>MKIGVIGAGTMGQGIAKAFAQVEGNTVALCDIKQEWAENGLAKIKKGYEKLVAKGKIPQEKADAIVAAITPGLKENLCADCDLIVEAAFEDMKVKQTTFGELDKICKPECIFASNTSSLSITEIGKGLSRPLVGMHFF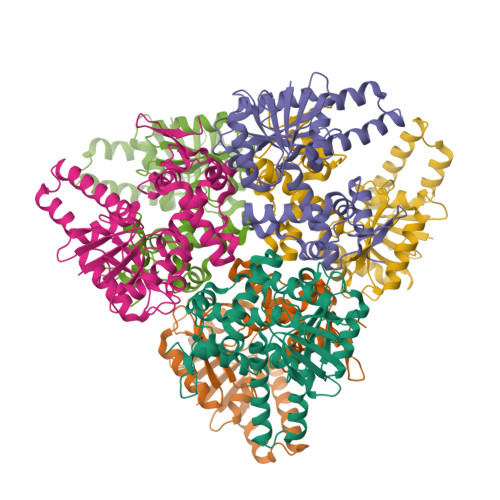NPADRMKLIEVIAGCNTPAETVEKIKEISVAIGKNPVQVNEAAGFVVNRILIPMINEAAFIKMEGVSDIAGIDTAMKLGANHPMGPLELGDFIGLDICLAIMDVLYHETGDSKYRACPLIRKMVRGGNLGCKTGKGFYVYNADRTKTPVDQL[6x]> GWVWNQFFVIEEYTGPDPVLVGRLHSDIDSGDGNIKYILSGEGAGTIFVIDDKSGNIHATKTLDREERAQYTLMAQAVDRDTNRPLEPPSEFIVKVQDINDNEPIFTKDVYTATVPEMADVGTFVVQVTATDADDPTYGNSAKVVY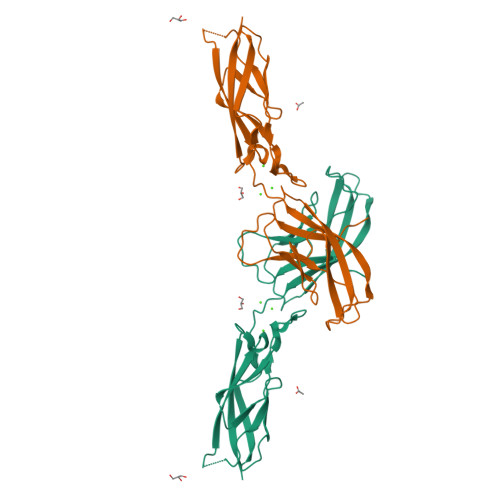SILQGQPYFSVESETGIIKTALLNMDRENREQYQVVIQAKDMGGQMGGLSGTTTVNITLTD> MERYENLFAQLNDRREGAFVPFVTLGDPGIEQSLKIIDTLIDAGADALELGVPFSDPLADGPTIQNANLRAFAAGVTPAQCFEMLALIREKHPTIPIGLLMYANLVFNNGIDAFYARCEQVGVDSVLVADVPVEESAPFRQAALRHNIAPIFICPPNADDDLLRQVASYGRGYTYLLSRSGVTGAENRGALPLHHLIEKLKEYHAAPALQGFGISSPEQVSAAVRAGAAGAISGSAIVKIIEKNLASPKQMLAELRSFVSAMKAASRA;> MTTLLNPYFGEFGGMYVPQILMPALNQLEEAFVRAQKDPEFQAQFADLLKNYAGRPTALTKCQNITAGTRTTLYLKREDLLHGGAHKTNQVLGQALLAKRMGKSEIIAETGAGQHGVA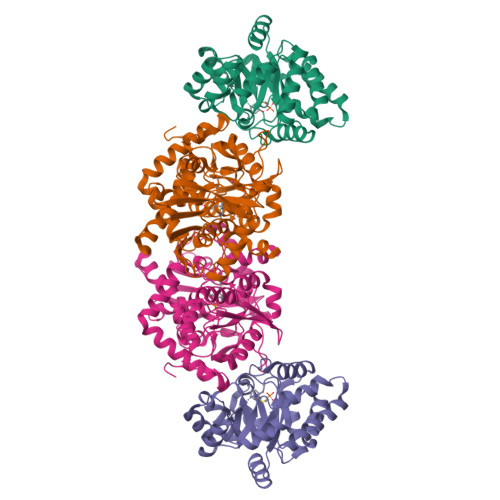SALASALLGLKCRIYMGAKDVERQSPNVFRMRLMGAEVIPVHSGSATLKDACNEALRDWSGSYETAHYMLGTAAGPHPYPTIVREFQRMIGEETKAQILDKEGRLPDAVIACVGGGSNAIGMFADFINDTSVGLIGVEPGGHGIETGEHGAPLKHGRVGIYFGMKAPMMQTADGQIEESYSISAGLDFPSVGPQHAYLNSIGRADYVSITDDEALEAFKTLCRHEGIIPALESSHALAHALKMMREQPEKEQLLVVNLSGRGDKDIFTVHDILKARGEI> MAEIPKEMLRAQTNVILLNVLKQGDNYVYGIIKQVKEASNGEMELNEATLYTIFKRLEKD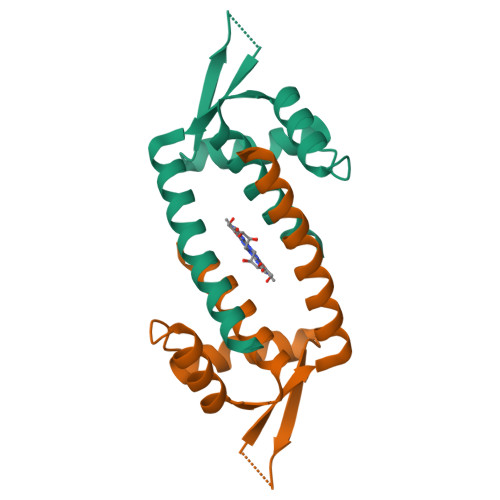GIISSYWGDESQGGRRKYYRLTEIGHENMRLAFESWSRVDKIIENLEANKKSEAIK>[2x]GLECDGKVNICCKKQFFVSFKDIGWNDWIIAPSGYHANYCEGECPSHIAGTSGSSLSFHSTVINHYRMRGHSPFANLKSCCVPTKLRPMSMLYYDDGQNIIKKDIQNMIVEECGCS;>[2x]GNCWLRQAK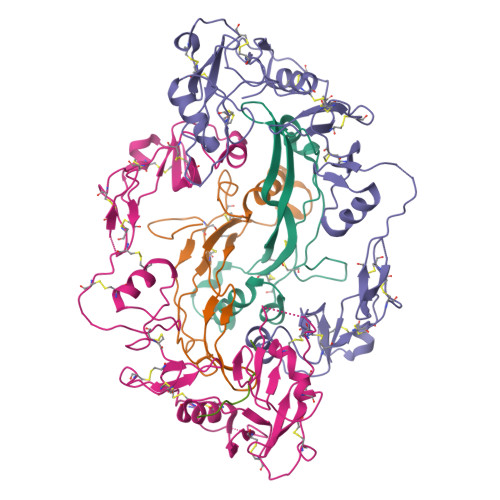NGRCQVLYKTELSKEECCSTGRLSTSWTEEDVNDNTLFKWMIFNGGAPNCIPCKETCENVDCGPGKKCRMNKKNKPRCVCAPDCSNITWKGPVCGLDGKTYRNECALLKARCKEQPELEVQYQGRCKKTCRDVFCPGSSTCVVDQTNNAYCVTCNRICPEPASSEQYLCGNDGVTYSSACHLRKATCLLGRSIGLAYEGKCIKAKSCEDIQCTGGKKCLWDFKVGRGRCSLCDELCPDSKSDEPVCASDNATYASECAMKEAACSSGVLLEVKHSGSCNSISEDTEEEEEDEDQDYSFPISSILEW;> AAAAAAAAAA N-{2-[1-(6-carbamoylthieno[3,2-d]pyrimidin-4-yl)piperidin-4-yl]ethyl}-N'-ethylthiophene-2,5-dicarboxamide 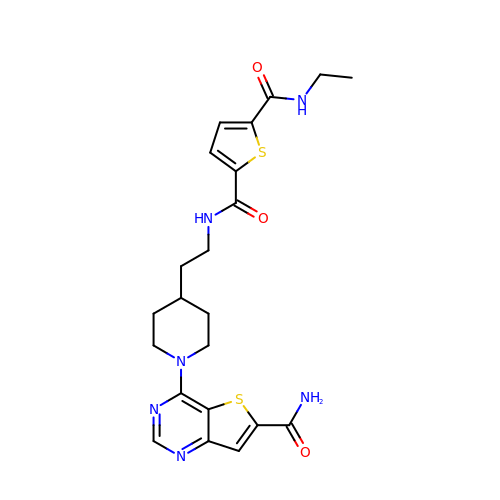| C22 H26 N6 O3 S2 | IXDTWYVAYLILOL-UHFFFAOYSA-N>HHHHHHENLYFQGSETFQDKVNFFQRELRQVHMKRPHSKVTLKVSRHALLESSLKATRNFSISDWSKNFEVVFQDEEALDWGGPRREWFELICKALFDTTNQLFTRFSDNNQALVHPNPNRPAHLRLKMYEFAGRLVGKCLYESSLGGAYKQLVRARFTRSFLAQIIGLRMHYKYFETDDPEFYKSKVCFILNNDMSEMELVFAEEKYNKSGQLDKVVELMTGGAQTPVTNANKIFYLNLLAQYRLASQVKEEVEHFLKGLNELVPENLLAIFDENELELLMCGTGDISVSDFKAHA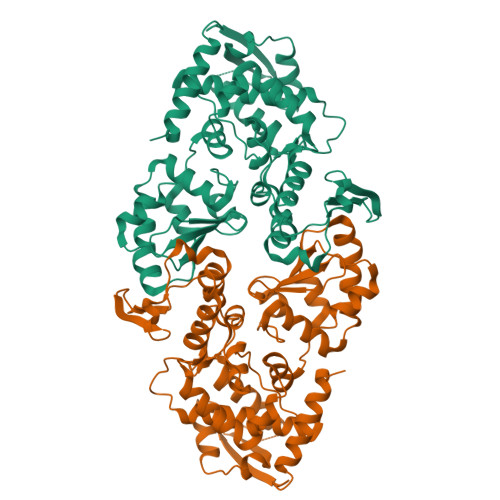VVVGGSWHFREKVMRWFWTVVSSLTQEELARLLQFTTGSSQLPPGGFAALCPSFQIIAAPTHSTLPTAHTCFNQLCLPTYDSYEEVHRMLQL[3x]> SDILGMLKSLHQLQVENRRLEEQIKNLTAKKERLQL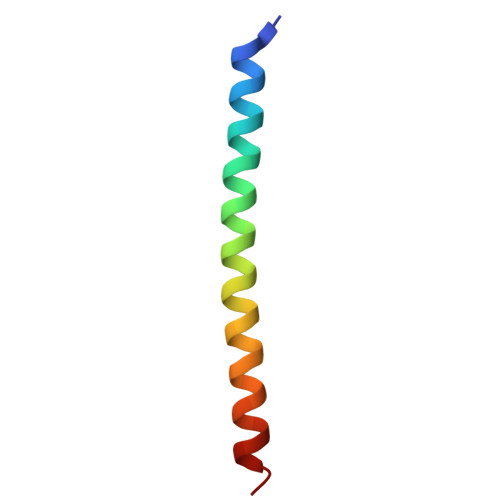LNAQLSV>MFDTSPRLDCAGRILTLDRPRVMGIVNVTPDSFSDGGTHTTVEAAVAHGLRLAEEGADLLDIGGESTRPGATAVPVEEELRRVIPVIERLVAQTALPLSVDTFKPEVMRAAVAAGAGMINDVQALRQPGALDAVADLRVPVVLMHMPGDAYAAGSAPHYDDVVAEVHRFLVERIFAAEMAGIDKRRLLIDPGFGFGKSTADNVQLLAHLPRLCELGVPVLAGLSRKRSIGELTGRELPEQRVAGSVAAHLLAAQRGALLLRVHDVAATV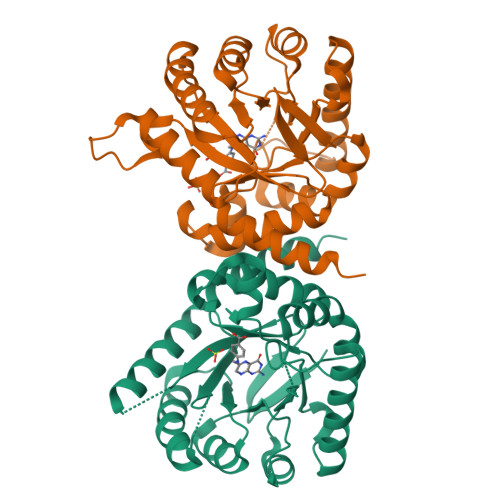DALTVWQAVQAVPSPRVATGTAMPIRWPDED[2x]>MEQTQKLKLNLQHFASNNVKPQVFNPDNVMMHEKKDGTLMNEFTTPILQEVMENSKIMQLGKYEPMEGTEKKFTFWADKPGAYWVGEGQKIETSKATWVNATMRAFKLGVILPVTKEFLNYTYSQFFEEMKPMIAEAFYKKFDEAGILNQGNNPFGKSIAQSIEKTNKVIKGDFTQDNIIDLEALLEDDELEANAFISKTQNRSLLRKIVDPETKERIYDRNSDSLDGLPVVNLKSSNLKRGELITGDFDKLIYGIPQLIEYKIDETAQLSTVKNEDGTPVNLFEQDMVALRATMHVALHIADDKAFAKLVPADKRTDSVPGEV[4x];>METKYELNNTKKVANAFGLNEEDTNLLINAVDLDIKNNMQEISSELQQSEQSKQKQYGTTLQNLAKQNRIIK[4x]

Like other tailed, double-stranded (ds) DNA bacteriophages (order Caudovirales), the 80α capsid protein (CP, 324 residues) is first assembled into an empty procapsid, requiring a scaffolding protein (SP, 206 residues), which acts as a chaperone for the assembly process. The CP models show the expected HK97-like fold common to the Caudovirales, divided into A- and P-domains, with an extended E-loop and an N-arm that folds along the inside of the P-domain. Many SaPIs also cause the redirection of the helper phage assembly pathway to form capsids that are smaller than those normally formed by the phage and are therefore unable to package complete phage genomes. For SaPI1, we previously demonstrated that this size redirection depended on the SaPI1-encoded proteins CpmA and CpmB, leading to the formation of a 45 nm diameter capsid with T = 4 icosahedral symmetry.

In the T = 4 SaPI1 procapsid, there are four subunits, organized as A5 pentamers and (BCD)2 hexamers, which superimpose with RMSD = 1.5–2.9 Å. These hexamers sit on the icosahedral twofold axes and thus have strict twofold symmetry. The SaPI1 procapsid map had the internal protrusions previously attributed to dimers of CpmB. Closer to the capsid shell, the density became interpretable, and was modeled de novo as residues 41–72 of CpmB. The C-terminal part of CpmB that includes the RIIK motif forms a helix-and-hook structure that is almost identical to that formed by SP in the 80α procapsid, and makes similar interactions with CP. Contacts between CpmB and adjacent CP subunits are more extensive than in the 80α procapsid, involving several additional Gln residues in the α-helix (Q48, Q51, Q56). Each CpmB dimer straddles two capsomers with legs that connect with the capsid shell. There are two types of protrusions: one that ties together C and D subunits around the threefold axis, and another, weaker density, that interacts with A and B subunits, connecting hexamers and pentamers around quasi-threefold symmetry axes. The small capsids have a more acute dihedral angle between capsomers, especially around the icosahedral threefold axis, where we previously showed that CpmB dimer occupancy was higher. CpmB dimers constrain these angles by straddling adjacent capsomers, whereas the longer, more flexible N-terminal domain of SP apparently does not constrain the capsomers in the same way.> MRRAAMYEEGPPPSYESVVSAAPVAAALGSPFDAPLDPPFVPPRYLRPTGGRNSIRYSELAPLFDTTRVYLVDNKSTDVASLNYQNDHSNFLTTVIQNNDYSPGEASTQTINLDDRSHWGGDLKTILHTNMPNVNEFMFTNKFKARVMVSRLPTKDNQVELKYEWVEFTLPEGNYSETMTIDLMNNAIVEHYLKVGRQNGVLESDIGVKFDTRNFRLGFDPVTGLVMPGVYTNEAFHPDIILLPGCGVDFTHSRLSNLLGIRKRQPFQEGFRITYDDLEGGNIPALLDVDAYQASLKDDTEQGGGGAGGSNSSGSGAEENSNAAAAAMQPVEDMNDHAIRGDTFATRAEEKRAEAEAAAEAAAPAAQPEVEKPQKKP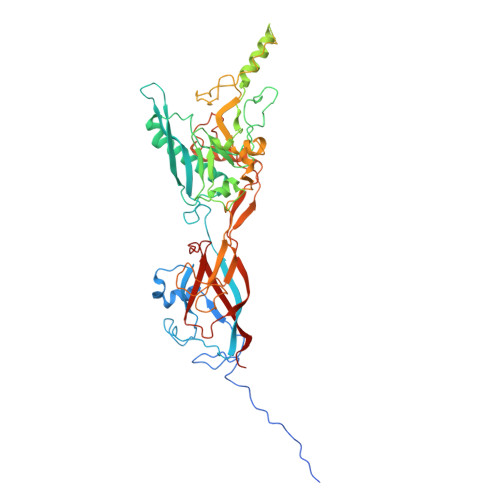VIKPLTEDSKKRSYNLISNDSTFTQYRSWYLAYNYGDPQTGIRSWTLLCTPDVTCGSEQVYWSLPDMMQDPVTFRSTRQISNFPVVGAELLPVHSKSFYNDQAVYSQLIRQFTSLTHVFNRFPENQILARPPAPTITTVSENVPALTDHGTLPLRNSIGGVQRVTITDARRRTCPYVYKALGIVSPRVLSSRTF>[3x]HHMAQANFGVVGMAVMGKNLALNVESRGYTVAIYNRTTSKTEEVFKEHQDKNLVFTKTLEEFVGSLEKPRRIMLMVQAGAATDATIKSLLPLLDIGDILIDGGNTHFPDTMRRNAELADSGINFIGTGVSGGEKGALLGPSMMPGGQKEAYDLVAPIFEQIAAKAPQDGKPCVAYMGANGAGHYVKMVHNGIEYGDMQLIAESYDLLKRILGLSNAEIQAIFEEWNEGELDSYLIEITKEVLKRK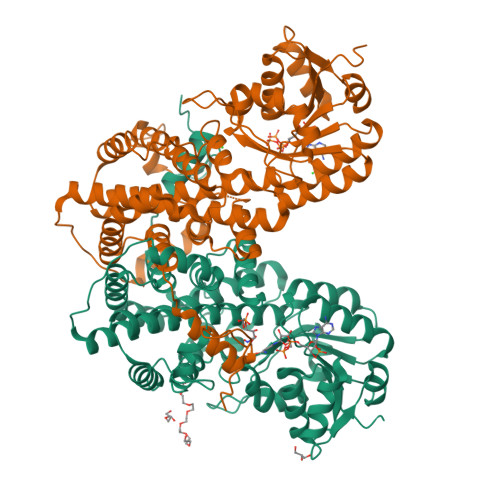DDEGEGYIVDKILDKAGNKGTGKWTSESALDLGVPLPLITESVFARYISTYKDERVKASKVLSGPALDFSGDKKEVIEKIRKALYFSKIMSYAQGFAQLRKASEEFDWDLPYGTIAQIWRAGCIIRAEFLQNITDAFDKDSELENLLLDDYFVDITKRYQEAVRDVVSLAVQAGTPIPTFTSAISYYDSYRSENLPANLIQAQRDYFGAHTYERTDKAGIFHYDWYTED>GSHMASSESTEEKPDTDLADKYASGNSEISGQELRGLRDAIGDDASPEDILALVQEKIKDPALQSTALDYLVQTTPPSQGKLKEALIQARNTHTEQFGRTAIGAKNILFASQEYADQLNVSPSGLRSLYLEVTGDTHTCDQLLSMLQDRYTYQDMAIVSSFLMKGMATGLKRQGPYVPSAQLQVLMTETRNLQAVLTSYDYFESRVPILLDSLKAEGIQTPSDLNFVKVAESYHKIINDKFPTASKVEREVRNLIGDDVDSVTGVLNLFFSALRQTSSRLFSSADKRQQLGAMIANALDAVNINNEDYPKASDFPKPYPWS[2x];>GSHMASMSHLNYLLEKIAASSKEDFPFPDDLESYLEGYVPDKNIALDTYQKIFKISSEDLEKVYKEGYHAYLDKDYAKSITVFRWLVFFNPFVSKFWFSLGASLHMSEQYSQALHAYGVTAVLRDKDPYPHYYAYICYTLTNEHEEAEKALEMAWVRAQHKPLYNELKEEILDIRKHK[2x]

The type three secretion (T3S) apparatus is a conserved molecular machine that forms a protein-conducting channel from the bacterial cytosol to the target cell cytosol. Our understanding of how the T3SS switches from translocator to effector secretion is limited, but in multiple systems this process is known to involve a conserved gatekeeper protein. Translocator-specific chaperones (class II chaperones) bind directly to translocators, prevent their degradation, and maintain the translocators in a secretion competent state. Protein delivery occurs in a highly regulated manner in which proteins involved in early steps in infection, or necessary to build the secretion conduit, are typically secreted before other substrates, a phenomenon termed secretion hierarchy. This study presents the structure of a molecular complex that physically links one class of early substrates, components of the secretion pore termed translocators, to a gatekeeper protein, a protein that has been implicated in the secretion hierarchy.

The amino terminal 84 residues of CopN were not included in the construct used for crystallization because they are unstructured. Two nearly identical Scc3-CopNΔ84 complexes (RMS deviation 0.34 Å for all CopNΔ84 mainchain atoms and 0.49 Å for all Scc3 mainchain atoms) are present in the asymmetric unit. CopNΔ84 forms a long cylindrical structure composed of three helical domains. CopNΔ84 is structurally similar to other gatekeeper proteins, both MxiC from Shigella and the YopN-TyeA complex from Yersinia. The structure reveals that Scc3 does not engage CopNΔ84 using this conserved binding groove. Instead, the amino terminus, referred to here as a gatekeeper-binding region (GBR), forms a relatively flat surface, adjacent to the convex side of the TPR and binds across the interdomain interface of the last two domains of CopNΔ84. The interface formed by this interaction results from burial of 980 Å2 of surface area. Residues 16–23 of Scc3 interact principally with site 1 of CopNΔ84, whereas residues 24–43 form a much larger interface in which Scc3 projects a ring of hydrophobic sidechains toward CopNΔ84 to surround a highly conserved arginine (R365) on CopNΔ84. This interaction includes three tyrosines, one of which, Y43 is oriented to allow a π-cation interaction. The Scc3-CopNΔ84 binding mode leaves the translocator-binding site on Scc3 unperturbed and available to bind translocators.(3S)-3-amino-4-oxo-4-[(4-phenylmethoxyphenyl)amino]butanoic acid | C17 H18 N2 O4 | 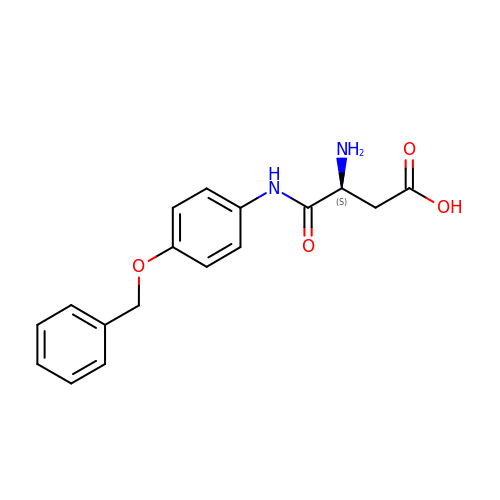VTMSXGVEMJOFRJ-HNNXBMFYSA-N>[2x]QLWRCQRQFLQHQRLRACQRFIHRRAQFGGQPD;>QPRRPALRQCCNQLRQVDRP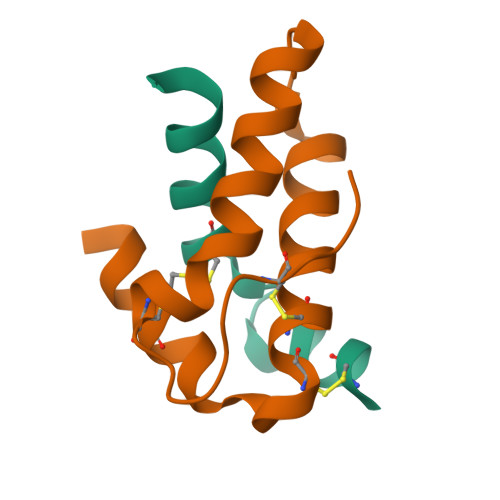CVCPVLRQAAQQVLQRQIIQGPQQLRRLFDAARNLPNICNIPNIGACPFRAW[2x]>MELWLVRHGETLWNREGRLLGWTDLPLTAEGEAQARRLKGALPSLPAFSSDLLRARRTAELAGFSPRLHPE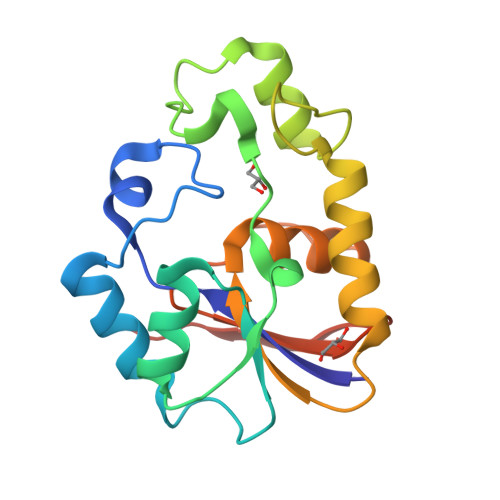LREIHFGALEGALWETLDPRYKEALLRFQGFHPPGGESLSAFQERVFRFLEGLKAPAVLFTHGGVVRAVLRALGEDGLVPPGSAVAVDWPRRVLVRLALDGEEATG[2x]Phosphoethanolamine (pEtN) cellulose is a naturally occurring modified cellulose produced by several Enterobacteriaceae. The minimal components of the E. coli cellulose synthase complex include the catalytically active BcsA enzyme, a hexameric semicircle of the periplasmic BcsB protein, and the outer membrane (OM)-integrated BcsC subunit containing periplasmic tetratricopeptide repeats (TPR). Additional subunits include BcsG, a membrane-anchored periplasmic pEtN transferase associated with BcsA, and BcsZ, a periplasmic cellulase of unknown biological function. Cellulose is a common bacterial biofilm component produced by a variety of prokaryotes, such as Escherichia coli (Ec), Salmonella enterica, and Gluconacetobacter/Komagataeibacter xylinus (Gx). These Gram-negative bacteria synthesize cellulose and secrete it across the cell envelope via the Bacterial cellulose synthase (Bcs) complex.

To our surprise, however, we discovered homo-oligomerization of the cellulase. Single particle cryo-EM analysis at a resolution of about 2.7 Å revealed the presence of BcsZ tetramers, in addition to small monomeric particles, Figs. 5d–f and S3g, S12e and Table S1. The homodimer interface is formed by helices 11 and 12 of the glycosylhydrolase-8 fold. It is rich in ionic interactions, including Asp344 and Arg318 of one protomer and the equivalent residues in the symmetry-related subunit. Combined, these interactions create a square-shaped tetrameric assembly with the cellulose-binding clefts of BcsZ subunits at opposing corners facing in the same direction. However, because BcsZ binds cellulose in a defined orientation, the 2-fold symmetry-related subunits bind their polymeric substrate in opposing directions, Fig. 5e. Oligomerization of BcsZ may optimize the enzyme’s ability to interact with and digest cellulose to increase catalytic efficiency, as frequently observed for carbohydrate-active enzymes. Collectively, our results indicate that cellulase activity is critical for cellulose export.

>MACTWPAWEQFKKDYISQEGRVIDPSDARKITTSEGQSYGMFSALAANDRAAFDNILDWTQNNLAQGSLKERLPAWLWGKKENSKWEVLDSNSASDGDVWMAWSLLEAGRLWKEQRYTDIGSALLKRIAREEVVTVPGLGSMLLPGKVGFAEDNSWRFNPSYLPPTLAQYFTRFGAPWTTLRETNQRLLLETAPKGFSPDWVRYEKDKGWQLKAEKTLISSYDAIRVYMWVGMMPDSDPQKARMLNRFKPMATFTEKNGYPPEKVDVATGKAQGKGPVGFSAAMLPFLQNRDAQAVQRQRVADNFPGSDAYYNYVLTLFGQGWDQHRFRFSTKGELLPDWGQECANSHLEHHHHHH[4x]> HHHHHHHHHHAQVNIAPGSLDKALNQYAAHSGFTLSVDASLTRGKQSNGLHGDYDVESGLQQLLDGSGLQVKPLGNNSWTLEPAPAPKEDALTVVGDWLGDARENDVFEHAGARDVIRREDFAKTGATTMREVLNRIPGVSAPENNGTGSHDLAMNFGIRGLNPRLASRSTVLMDGIPVPFAPYGQPQLSLAPVSLGNMDAIDVVRGGGAVRYGPQSVGGVVNFVTRAIPQDFGIEAGVEGQLSPTSSQNNPKETHNLMVGGTADNGFGTALLYSGTRGSDWREHSATRIDDLMLKSKYAPDEVHTFNSLLQYYDGEADMPGGLSRADYDADRWQSTRPYDRFWGRRKLASLGYQFQPDSQHKFNIQGFYTQTLRSGYLEQGKRITLSPRNYWVRGIEPRYSQIFMIGPSAHEVGVGYRYLNESTHEMRYYTATSSGQLPSGSSPYDRDTRSGTEAHAWYLDDKIDIGNWTITPGMRFEHIESYQNNAITGTHEEVSYNAPLPALNVLYHLTDSWNLYANTEGSFGTVQYSQIGKAVQSGNVEPEKARTWELGTRYDDGALTAEMGLFLINFNNQYDSN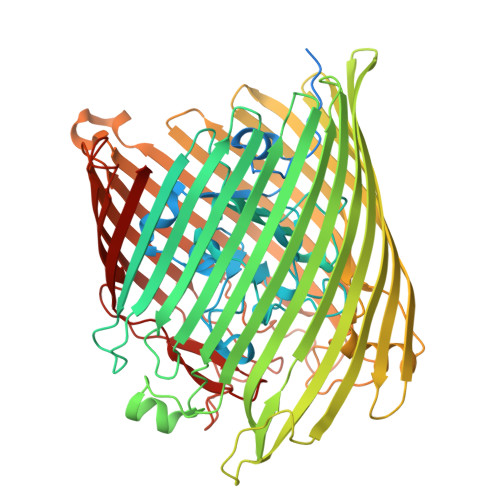QTNDTVTARGKTRHTGLETQARYDLGTLTPTLDNVSIYASYAYVNAEIREKGDTYGNLVPFSPKHKGTLGVDYKPGNWTFNLNSDFQSSQFADNANTVKESADGSTGRIPGFMLWGARVAYDFGPQMADLNLAFGVKNIFDQDYFIRSYDDNNKGIYAGQPRTLYMQGSLKF>SNAMHMQLKGKTALVTGSTAGIGKAIATSLVAEGANVLINGRREENVNETIKEIRAQYPDAILQPVVADLGTEQGCQDVIEKYPKVDILINNLGIFEPVEYFDIPDEDWFKLFEVNIMSGVRLTRSYLKKMIERKEGRVIFIASEAAIMPSQEMAHYSATKTMQLSLSRSLAELTTGTNV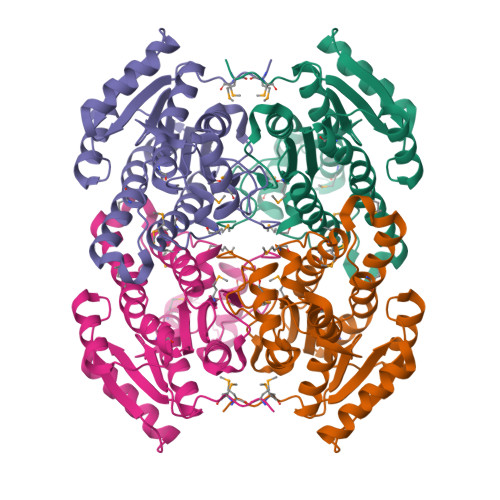TVNTIMPGSTLTEGVETMLNSLYPNEQLTIEEAEKRFMKENRPTSIIQRLIRPEEIAHLVTFLSSPLSSAINGSALRIDGGLVRSVF[2x]>[4x]MKVVKEFSVCGGRLIKLSHNSNSTKTSMNVNIYLPKHYYAQDFPRNKRIPTVFYLSGLTCTPDNASEKAFWQFQADKYGFAIVFPDTSPRGDEVANDP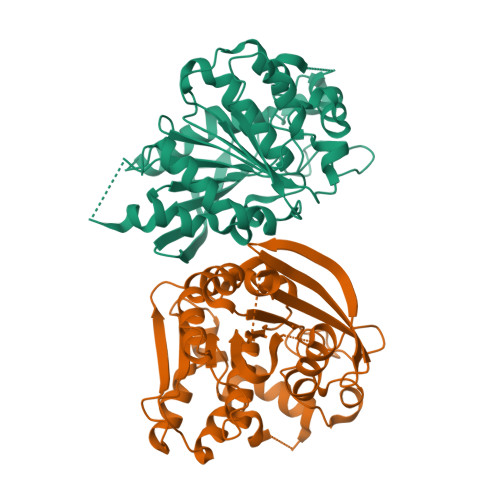EGSWDFGQGAGFYLNATQEPYAQHYQMYDYIHKELPQTLDSHFNKNGDVKLDFLDNVAITGISMGGYGAICGYLKGYSGKRYKSCSAFAPIVNPSNVPWGQKAFKGYLGEEKAQWEAYDPCLLIKNIRHVGDDRILIHVGDSDPFLEEHLKPELLLEAVKATSWQDYVEIKKVHGFDHSYYFVSTFVPEHAEFHARNLGLI> MRLKVKQSSANVHSELTAAVGWNVWNELFTCSDDQTIHKWNMLGEPEQKVSTLDAYFTDMHWYPVSSKKTQAGGTDVFAVACTDGSVKILSRTGRVEKSIEGHKGACISLRWSYDGTALATAGEDGSVKIWSRNGMLRSTLAQADSPVYSIVWAYDCDQLCYCTGSNVVIKSLSSNAKQNAWKAHDGVVLKVDWSPINHLIITGGEDCKYKVWDSFGRLLFQSGLFDYPVTSVAWAPSGELFAVGGFNTLQLCDRMGWAYSKIHLNDTGSIMTLSWTADSTQLAGGGGSGGVVFGQVVDLALEDGKMQVTVVDDMRIVVNDILNENADELPEFRDRVIKVSLGYGYLIVATATQCHVYNTTNLGTPHIFDLKDTVTLLLQAERHFLLLDNSAGIQIYTYEGRQICNPRFQGLRTELLNA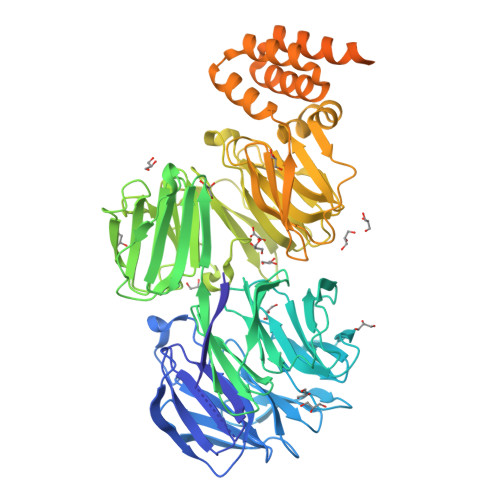QMITLSNDTIAVLDQQASGTTVRFFDTAQGRPVGEPWQHTLEVKEIALSQAGTINDRQLIVIDRNRDLYLLPVMKRHVAKLAAMCDSARWHDSTAMLSAMVDQRLCVWYYPSEVYVDKDLLAKTRYTKSDSDFGKSAQIQLFAGNRCLVRRSDGVLVSAATSPYPAVLYDMIRKQQWDKATRLCRFIKDPTMWATLAAMAMAAKELNTAEVAFAAIDEVDKTHFVRKVKQIPTEEGRNAELAVYRRKPEEGESILLQAGLVFRAIKLNIKLFNWERALDLATQHKQHQDTVLWYRQQFLKNAKLAESITRFMQMNESVVVDQAAVKKKIEEERIKESQRPGAKRYVHHHHHH>[3x]MAHHHHHHMTAYRIAPSILSADFARLGEEVANVIAAGADLIHFDVMDNHYVPNLTFGPMVCAALKPYASVPIDVHLMVEPVDDLIQSFAKAGASIITFHPEASRHI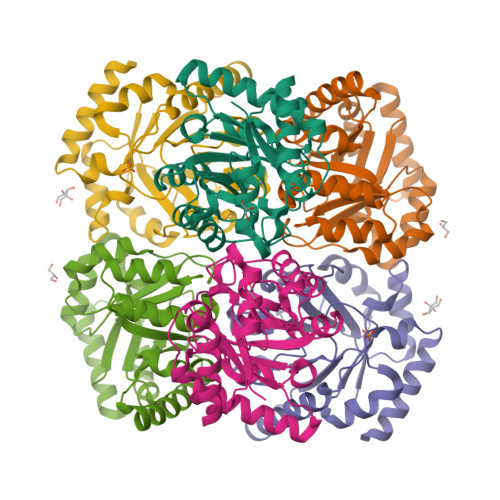DRSLSLIRDMGCQAGLVLNPATPVYVLENVLDRLDMVLLMSVNPGFGGQSFIPHTLEKIRQVRAMLDRYEGKSGRRIAIEVDGGIKTDNIAAVARAGADTFVAGSAIFGKPDYKAVIAAMRAELEKAAG> MAAPVVAPPGVVVSRANKRSGAGPGGSGGGGARGAEEEPPPPLQAVLVADSFDRRFFPISKDQPRVLLPLANVALIDYTLEFLTATGVQETFVFCCWKAAQIKEHLLKSKWCRPTSLNVVRIITSELYRSLGDVLRDVDAKALVRSDFLLVYGDVISNINITRALEEHRLRRKLEKNVSVMTMIFKESSPSHPTRCHEDNVVVAVDSTTNRVLHFQKTQGLRRFAFPLSLFQGSSDGVEVRYDLLDCHISICSPQVAQLFTDNFDYQTRDDFVRGLLVNEEILGNQIHMHVTAKE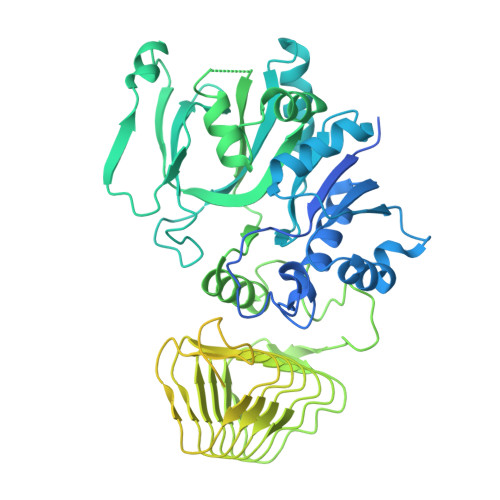YGARVSNLHMYSAVCADVIRRWVYPLTPEANFTDSTTQSCTHSRHNIYRGPEVSLGHGSILEENVLLGSGTVIGSNCFITNSVIGPGCHIGDNVVLDQTYLWQGVRVAAGAQIHQSLLCDNAEVKERVTLKPRSVLTSQVVVGPNITLPEGSVISLHPPDAEEDEDDGEFSDDSGADQEKDKVKMKGYNPAEVGAAGKGYLWKAAGMNMEEEEELQQNLWGLKINMEEESESESEQSMDSEEPDSRGGSPQMDDIKVFQNEVLGTLQRGKEENISCDNLVLEINSLKYAYNVSLKEVMQVLSHVVLEFPLQQMDSPLDSSRYCALLLPLLKAWSPVFRNYIKRAADHLEALAAIEDFFLEHEALGISMAKVLMAFYQLEILAEETILSWFSQRDTTDKGQQLRKNQQLQRFIQWLKEAEEESSEDD>MDQNFARNEKEAKDSAITFIQKSAAIKAGARSAEDIKLDKVNLGGELSGSNMYVYNISTGGFVIVSGDKRSPEILGYSTSGSFDANGKENIASFMESYVEQIKENKKLDTTYAGTAEIKQPVVKSLLNSKGIHYNQGNPYNLLTPVIEKVKPGEQSFVGQHAATGCVATATAQIMKYHNYPNKGLKDYTYTLSSNNPYFNHPKNLFAAISTRQYNWNNILPTYSGRESNVQKMAISELMADVGISVDMDYGPSSGSAGSSRVQRALKENFGYNQSVHQINRSDFSKQ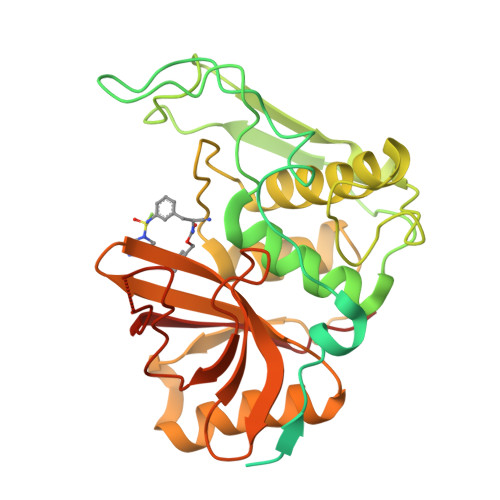DWEAQIDKELSQNQPVYYQGVGKVGGHAFVIDGADGRNFYHVNWGWGGVSDGFFRLDALNPSALGTGGGAGGFNGYQSAVVGIKPLEHHHHHH[2x]> MFLRTHVERHRSGKARAFVFRDPTLKMMRAGSGYQQLRRMGMPIQVSKGWRKVDHFHANNQYQHAWPLLSHDDLGNSDQSNNTRNIMYSMYLPKRNKGTAPWFRGADTYSVKYCEQGRYEYQRYLMINRFPSEYRKHFMNFLSNIRSSSGPATIPQEALHWLLRMIVDNFNPQHVHYIAAMKTLQNAGELDMARDVWKIMERQQTWPCTSTICAYLDVCVEAGEKTWAMEAWNRYCTELKFLQPGEVDPKPVSRVPFSLTREELLYLPKWKKHFDHDPNLDVVDLNRFNRTREVYLRMAQVMLAGGERDSFQHFYTKLEEAMLSTPTPVPEPPNPHLVRRPQWSPYEHCKSVHHSPWRVGNNGRAMALGPSLTTEDEMQSRFFSNDQFLVHMLKEILRIVLQEHRRRHPEACSRGEGEAFFDQVVDARETLNFCNELIERLFAVLGQKMHGLNTSSLLSVILELYRVMGKETGMALLRRANQFLERKAALEDGAKESLTAPNYLQVLMGFADESA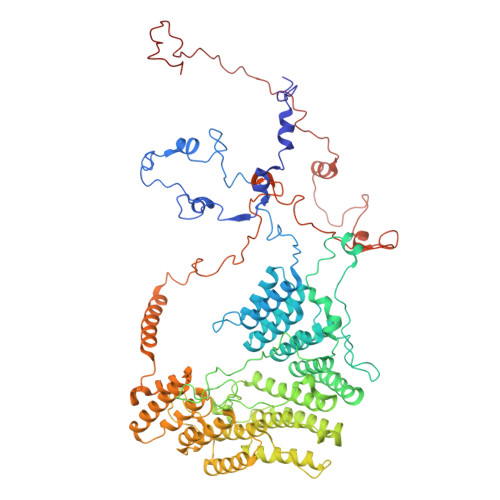YVYDSKRKGLCRYRSGFDPRTTMQQLAATVQEIAGNPHVTWAADMHLQVVCTMVGCGTMKANDYFVRNVLRQFCWDSRFLEALYMEYRRHDDVDMWAELTKRALVWTARYNVNASERLKRLIEDDYDTIQVHTRTFRELAVFQFRDVEEKRHSRDVVNELPNPWTDYVSHALPFPDRDAGYPDEYGDIGQWRAPGGPGSPVKGPGYYAPPMEGEHQRGYTAEWRDLKNPMRPPEFPTPWERKYKQYARGQHPSYDMVYAGPMPEIFPNRYDFRKPTRWDFHDIEKQGKYKTSGPY> MAASVEQREGTIQVQGQALFFREALPGSGQARFSVLLLHGIRFSSETWQNLGTLHRLAQAGYRA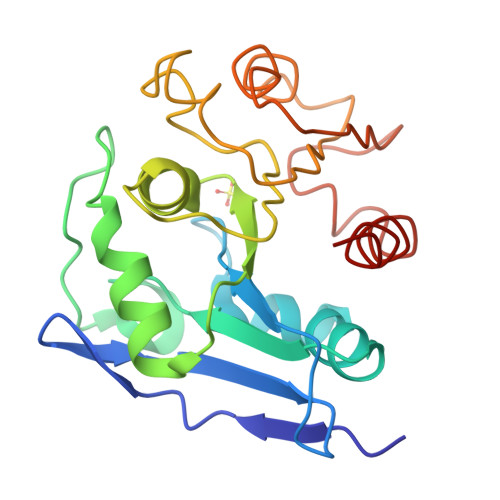VAIDLPGLGHSKEAAAPAPIGELAPGSFLAAVVDALELGPPVVISPSLSGMYSLPFLTAPGSQLPGFVPVAPICTDKINAANYASVKTPALIVYGDQDPMGQTSFEHLKQLPNHRVLIMKGAGHPCYLDKPEEWHTGLLDFLQGLQ> MKVNNTIVVSIGQAGNQIAASFWKTVCLEHGIDPLTGQTAPGVAPRGNWSSFFSKLGESSSGSYVPRAIMVDLEPSVIDNVKATSGSLFNPANLISRTEGAGGNFAVGYLGAGREVLPEVMSRLDYEIDKCDNVGGIIVLHAIGGGTGSGFGALLIESLKEKYGEIPVLSCAVLPSPQVSSVVTEPYNTVFALNTLRRSADACLIFDNEALFDLAHRKWNIESPTVDDLNLLITEALAGITASMRFSGFLTVEISLRELLTNLVPQPSLHFLMCAFAPLTPPDRSKFEELGIEEMIKSLFDNGSVFAACSPMEGRFLSTAVLYRGIMEDKPLADAALAAMREKLPLTYWIPTAFKIGYVEQPGISHRKSMVLLANNTEIARVLDRIC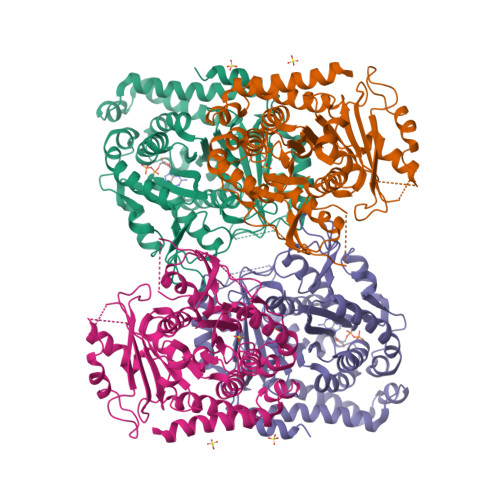HNFDKLWQRKAFANWYLNEGMSEEQINVLRASAQELVQSYQVAEESGAKAKVQDSAGDTGMRAAAAGVSDDARGSMSLRDLVDRRR;> VREILSIHVGQCGNQIADSFWRLALREHGLTEAGTLKEGSNAAANSNMEVFFHKVRDGKYVPRAVLVDLEPGVIARIEGGDMSQLFDESSIVRKIPGAANNWARGYNVEGEKVIDQIMNVIDSAVEKTKGLQGFLMTHSIGGGSGSGLGSLILERLRQAYPKKRIFTFSVVPSPLISDSAVEPYNAILTLQRILDNADGAVLLDNEALFRIAKAKLNRSPNYMDLNNIIALIVSSVTASLRFPGKLNTDLSEFVTNLVPFPGNHFLTASFAPMRGAGQEGQVRTNFPDLARETFAQDNFTAAIDWQQGVYLAASALFRGDVKAKDVDENMATIRKSLNYASYMPASGGLKLGYAETAPEGFASSGLALVNHTGIAAVFERLIAQFDIMFDNHAYTHWYENAGVSRDMMAKARNQIATLAQSYRDAS> GSHMASPNGQTKPLPALKLALEYIVPCMNKHGICVVDDFLGKETGQQIGDEVRALHDTGKFTDGQLVSQKSDSSKDIRGDKITWIEGKEPGC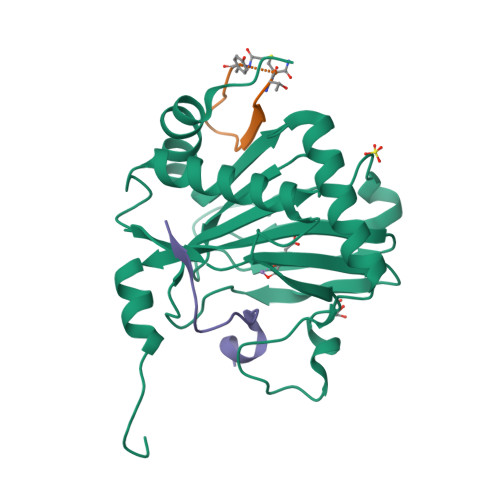ETIGLLMSSMDDLIRHCNGKLGSYKINGRTKAMVACYPGNGTGYVRHVDNPNGDGRCVTCIYYLNKDWDAKVSGGILRIFPEGKAQFADIEPKFDRLLFFWSDRRNPHEVQPAYATRYAITVWYFDADERARAKVKYLTGE;> XYVWLTDTWVLSRT;> DLDLEMLAPYIPMDDDFQL>[6x]MPG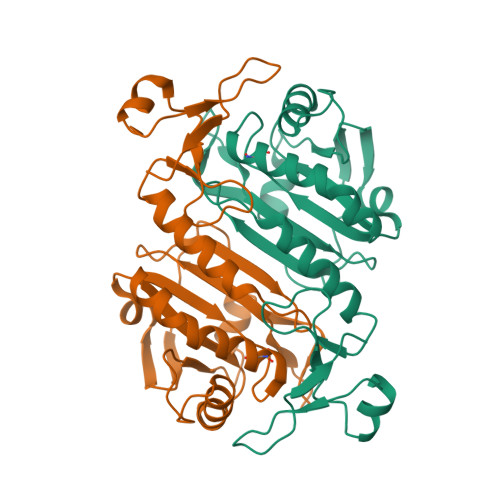GLLLGDVAPNFEANTTVGRIRFHDFLGDSWGILFSHPRDFTPVCTTELGRAAKLAPEFAKRNVKLIALSIDSVEDHLAWSKDINAYNCEEPTEKLPFPIIDDRNRELAILLGMLDPAEKDEKGMPVTARVVFVFGPDKKLKLSILYPATTGRNFDEILRVVISLQLTAEKRVATPVDWKDGDSVMVLPTIPEEEAKKLFPKGVFTKELPSGKKYLRYTPQP> MSTAVQFRGGTTAQHATFTGAAREITVDTDKNTVVVHDGATAGGFPLARHDLVKTAFIKADKSAVAFTRTGNATASIKAGTIVEVNGKLVQFTADTAITMPALTAGTDYAIYVCDDGTVRADSNFSAPTGYTSTTARKVGGFHYAPGSNAAAQAGGNTTAQINEYSLWDIKFRPAALDPRGMTLVAGAFWADIYLLGVNHLTDGTSKYNVTIA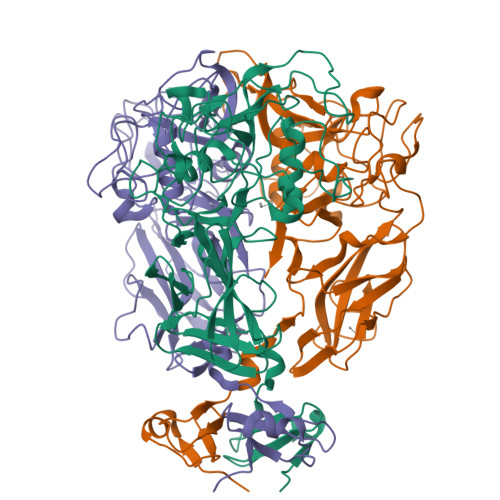DGSASPKKSTKFGGDGSAAYSDGAWYNFAEVMTHHGKRLPNYNEFQALAFGTTEATSSGGTDVPTTGVNGTGATSAWNIFTSKWGVVQASGCLWTWGNEFGGVNGASEYTANTGGRGSVYAQPAAALFGGNWSNTSHSGSRAALWYVGPSNSFAGIGARGVCDHLILE> MGTTTCKQCANFFP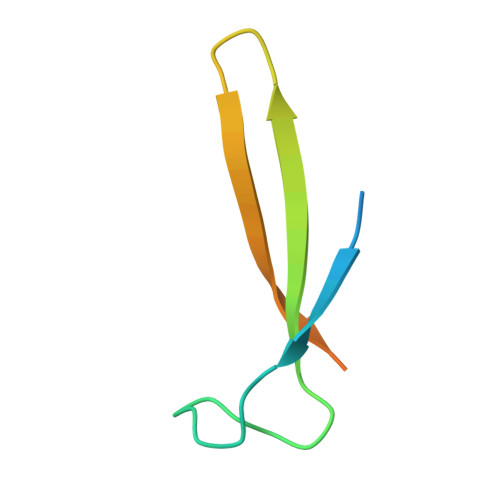VPKDADDYEAGKADCVREKEDEKGKYWLSKPIFENSAQCEAFQTKR>[4x]MERLWKDIKRDWLLYAMLLPTIIWFLIFLYKPMIGLQMAFKQYSAWKGIAGSPWIGFDHFVTLFQSEQFIRAIKNTLTLSGLSLLFGFPMPILLALMINEVYSKGYRKAVQTIVYLPHFISIVIVAGLVVTFLSPSTGVVNNMLSWIGLDRVYFLTQPEWFRPIYISSNIWKEAGFDSIVYLAAIMSINPALYESAQVDGATRWQMITRITLPCIVPTIAVLLVIRLGHILEVGFEYIILLYQPTTYETADVISTYIYRLGLQGARYDIATAAGIFNAVVALVIVLFANHMSRRITKTGVF;>[4x]MLATPFYSRSDRIFGIVNAVLLGIFALCALYPIIYIFSMSISSGAAVTQGRVFLLPVDIDFSAYGRVLHDKLFWTSYANTIFYTVFGVVTSLIFIVPGAYALSKPRIRGRRVFGFIIAFTMWFNAGMIPFFLNMRDLGLLDNRFGILIGFACNAFN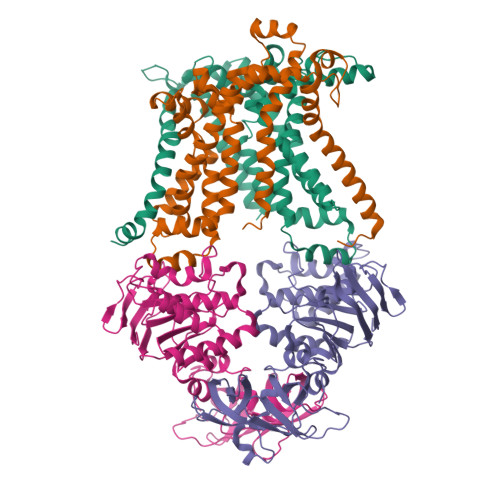IILMRNYFESISASFEEAARMDGANDLQILWKVYIPLAKPALATITLLCAISRWNGYFWAMVLLRAEEKIPLQVYLKKTIVDLNVNEEFAGALLTNSYSMETVVGAIIVMSIIPVIIVYPVVQKYFTKGVMLGGVKELEHHHHHHHHHH;>MVASVSIQNVVKRYDKTTVVHGVSLDIEPGEFVVLVGPSGCGKSTTLRMVAGLEEISGGTIRIDGRVINDLAPKDRDVAMVFQNYALYPHLNVRDNISFGLRLKRTKKSVIDAAVKTAADILGLQPLLERKPSDLSGGQRQRVAMGRAIVRDPKVFLFDQPLSNLDAKLRTQMRAEIKRLHQRLGTTVIYVTHDQVEAMTLADRIVVMRDGLIEQIGKPMDLFLHPANTFVASFIGSPPMNLMPARIAVDSTQHVELNGGNRISLLPRAGTHLAPGQEVVFGIRPEDVTLDGVEGSERAQIKATVDIVEPLGSESILHATVGDHSLVVKVGGLNEVHPGDPVTLHVDLTRVHLFDAQSQASIY[8x]>ALYEDPPDQKTSPSGKPATLKICSWNVDGLRAWIKKKGLDWVKEEAPDILCLQETKCSENKLPAELQELPGLSHQYWSAPSDKEGYSGVGLLSRQAPLKVSYGIGDEEHDQEGRVIVAEFDSFVLVTAYVPAAGRGLVRLEYRQRWDEAFRKFLKGLASRKPLVLCGDLNVAHEEIDLRNPKGNKKNAGFTPQERQGFGELLQAVPLADSFRHLYPNTPYAYTFWTYMMNARSKNVGWRLDYFLLSHSLLPALCDSKIRSKALGSDHCPITLYLAL[2x]

AP sites are then processed by apurinic/apyrimidinic endonuclease 1 (APE1), which cleaves the phosphodiester DNA backbone at the 5′ end of the AP site using its endonuclease activity. Upon binding an AP site, APE1 flips the AP site out of the DNA double helix and into an extrahelical position within the compact APE1 active site. In the human APE1 substrate complex, N174 is within hydrogen bonding distance of N212 and the AP site bridging oxygen (O5) and deoxyribose sugar oxygen (O4). To assess the role of N174 during APE1 catalysis, we rationally designed four mutations of N174: N174A, N174D, N174Q, and N174K.

The APE1N174A mutant had a kobs of 0.039 ± 0.003 s−1, corresponding to a 22,000-fold reduction in kobs compared to APE1WT. To test this, we crystallized the APE1N174A mutant protein bound to a 21-mer dsDNA oligo containing a centrally located THF AP site analog. This substrate complex diffracted to 2.29 Å resolution in the P1 space group. Overlay of the APE1WT and APE1N174A substrate complexes revealed similar active sites, with no notable differences in the position of key active site residues (RMSD = 0.299 of 2199 atoms). In contrast, shifts to the DNA within the active site are observed, with the AP site, phosphate backbone, and surrounding DNA adopting a different position in the APE1N174A mutant compared to APE1WT. Specifically, the AP site phosphate group is shifted 1.1 Å out of the APE1 active site in the APE1N174A mutant compared to APE1WT. This shift increases the distance between the phosphate of the AP site and the nucleophilic water, ultimately resulting in misalignment of the phosphate backbone for attack by the nucleophilic water. Based on these results, we conclude that the N174A mutation compromises hydrogen bonding between residue 174 and O4 and O5 of the AP site. Therefore, in APE1WT, the hydrogen bonds between N174 and the AP site are necessary to position the phosphate backbone of the AP site within the APE1 active site to support nucleophilic attack during catalysis.>[4x]MMKIKPVKVESIENPKRFLNSRLLTKIEVEEAIEKALKQLYINIDY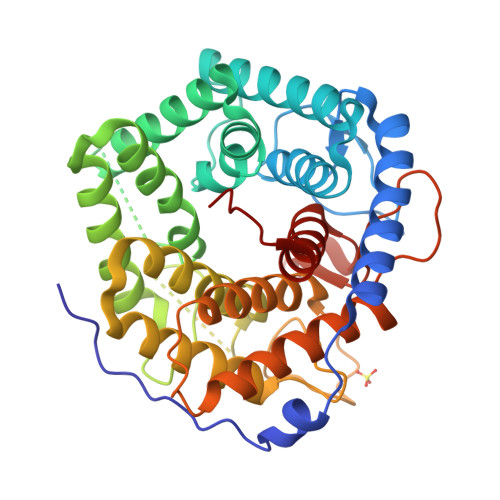FGEEYPTPATFNNIYKVMDNTEWTNGFWTGCLWLAYEYNQDKKLKNIAHKNVLSFLNRINNRIALDHHNLGFLYTPSCTAEYRINGDVKALEATIKAADKLMERYQEKGGFIQAWGELGYKEHYRLIIDCLLNIQLLFFAYEQTGDEKYRQVAVNHFYASANNVVRDDSSAFHTFYFDPETGEPLKGVTRQGYSDESSWARGQAWGIYGIPLSYRKMKDYQQIILFKGMTNYFLNRLPEDKVSYWDLIFTDGSGQPRDTSATATAVCGIHEMLKYLPEVDPDKETYKYAMHTMLRSLIEQYSNNELIAGRPLLLHGVYSWHSGKGVDEGNIWGDYYYLEALIRFYKDWELYW Cowpea mosaic virus (CPMV) is a plant-infecting member of the order Picornavirales, with a relatively simple, non-enveloped capsid that has been extensively studied. CPMV has an icosahedral capsid structure, which is ~30 nm in diameter and is formed from 60 copies each of a Large (L) and Small (S) coat protein. Crystallographic structures are available for three Comoviruses: CPMV, BPMV and red clover mottle virus. Together, the L and S subunits comprise three β-barrel domains (two from L, one from S) each of which contains a ‘jelly roll’ topology.

Until now there has been no individual structural analysis of CPMV-T and the RNA packaged into CPMV-M has not been visualised. Here we show high resolution cryo-EM structures of CPMV-M and CPMV-T to 3.9 Å and 4.2 Å respectively. The cryo-EM structures are of sufficient resolution to visualise the individual amino acid side chains and both structures reveal differences between the CPMV particles. The resolution of the map permits the side chains of the large amino acids to be visualised. EM density for S subunit residues 184 to 189 inclusive were not visible; these residues were removed from the model.

> GPVCAEASDVYSPCMIASTPPAPFSDVTAVTFDLINGKITPVGDDNWNTHIYNPPIMNVLRTAAWKSGTIHVQLNVRGAGVKRADWDGQVFVYLRQSMNPESYDARTFVISQPGSAMLNFSFDIIGPNSGFEFAESPWANQTTWYLECVATNPRQIQQFEVNMRFDPNFRVAGNILMPPFPLSTETPPL;> MEQNLFALSLDDTSSVRGSLLDTKFAQTRVLLSKAMAGGDVLLDEYLYDVVNGQDFRATVAFLRTHVITGKIKVTATTNISDNSGCCLMLAINSGVRGKYSTDVYTICSQDSMTWNPGCKKNFSFTFNPNPCGDSWSAEMISRSRVRMTVICVSGWTLSPTTDVIAKLDWSIVNEKCEPTIYHLADCQNWLPLNRWMGKLTFPQGVTSEVRRMPLSIGGGAGATQAFLANMPNSWISMWRYFRGELHFEVTKMSSPYIKATVTFLIAFGNLSDAFGFYESFPHRIVQFAEVEEKCTLVFSQQEFVTAWSTQVNPRTTLEADGCPYLYAIIHDSTTGTISGDFNLGVKLVGIKDFCGIGSNPGIDGSRLL>MASMTGGQQMGRDEAGITGTWYNQLGSTFIVTAGADGALTGTYESAAGKAESRYVLTGRYDSAPATDGSGTALGWTVAWKNNYRNAHSATTWSGQYVGGAEARINTQWLLTIGATEANGWASTYVGHDTFTKVKPSAASIDAAKKAGVNNGNPLDAVQQ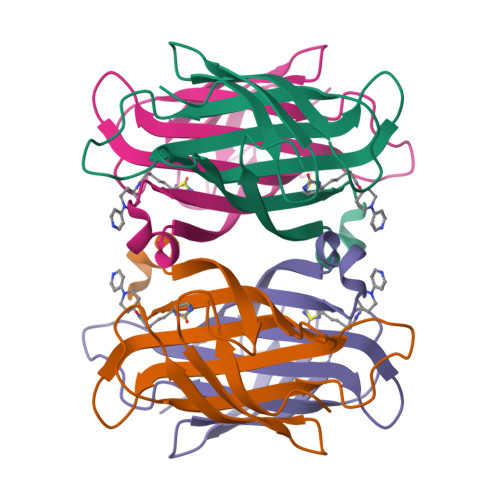[2x]> MGSSHHHHHHSSGENLYFQGHMAAPFDKSRNVAQSIDQLIGQTPALYLNKLNNTKAKVVLKMECENPMASVKDRLGFAIYDKAEKEGKLIPGKSVVV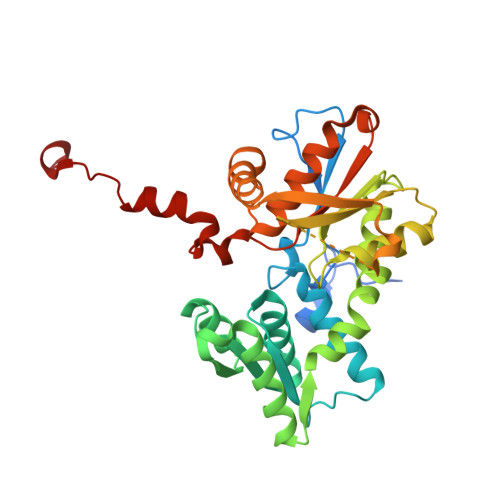ESSSGNTGVSLAHLGAIRGYKVIITMPESMSLERRCLLRIFGAEVILTPAALGMKGAVTMAKKIVTANPNAVLADQFATKYNALIHEETTGPEIWEQTNHNVDCFIAGVGTGGTLTGVARALKKMGSHARIVAVEPMESPVLSGGKPGAHKIQGIGPGFVPDVLDRSLIDEVFCVAGDDAIETALKLTRSDGVFCGFSGGANVYAALKIAERPEMEGKTIVTIIPSFGERYLSTALYRSVRDEVSSLPVVDASELQD> PRTIAEMRKEEMAKEMDPEKLKILEWIEGKERNIRALLSTMHTVLWAGETKWKPVGMADLV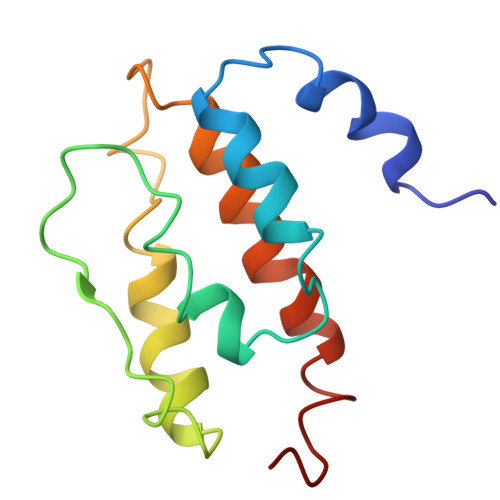TPEQVKKVYRKAVLVVHPDKATGQPYEQYAKMIFMELNDAWSEFENQGQKPLY> TQVLFEHPLNEKMRTWLRIEFLIQQLSINLPIADHAGALHFFRNISDLLDVFERGEVRTELLKELERQQRKLQAWVEVPGVDQDRIEALRQQLKSAGSVLISAPRIGQQLREDRLIALVRQRLSIPGGCCSFDLPTLHIWLHLQQAQRDAQIESWLASLNPLTQALTLVLDLIRNSAPFRKQTSLNGFYQDNGDDADLLRLMLTLDSQLYPQISGHKSRFAIRFMPLDSENGLVPERLDF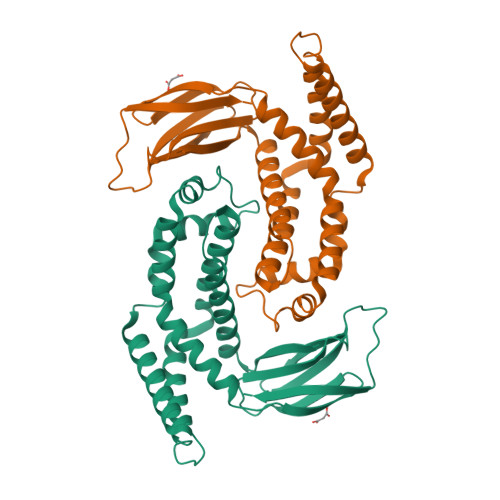ELACC> TGDERFYAEHLMPTLQGLLDPESAHRLAVRFTSLGLLPRARFQDSDMLEVRVLGHKFRNPVGIAAGFDKHGEAVDGLYKMGFGFVEIGSVTPKPQEGNPRPRVFRLPEDQAVINRYGFNSHGLSVVEHRLRARQQKQAKLTEDGLPLGVNLGKNKTSVDAAEDYAEGVRVLGPLADYLVVNVSSPNTAGLRSLQGKAELRRLLTKVLQERDGLRRVHRPAVLVKIAPDLTSQDKEDIASVVKELGIDGLIVTNTTVSRPAGLQGALRSETGGLSGKPLRDLSTQTIREMYALTQGRVPIIGVGGVSSG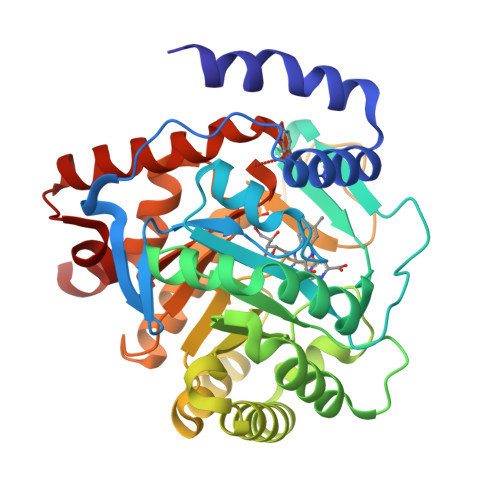QDALEKIRAGASLVQLYTALTFWGPPVVGKVKRELEALLKEQGFGGVTDAIGADHRR> EDPVTGPEEVSGQEQGSLTVQCRYT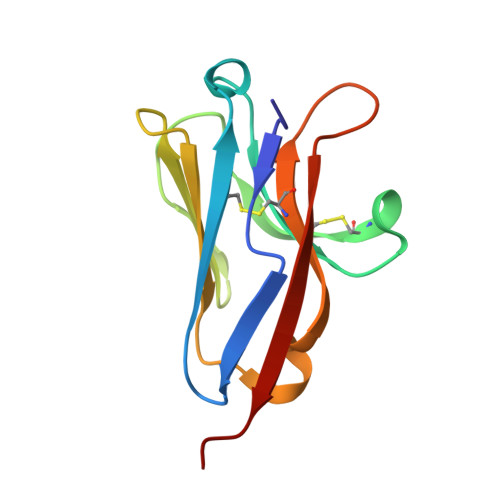SGWKDYKKYWCQGVPQRSCKTLVETDASEQLVKKNRVSIRDNQRDFIFTVTMEDLRMSDAGIYWCGITKGGLDPMFKVTVNIGPVP> GMRIPLVGKEPIEAEDMGFTLIHEHLRVFSEAVRYQWPHLYNEDEELRNAVNEVKRAMQFGVKTIVDPTVMGLGRDIRFMEKVVKTTGINLVAGTGIYIYVDLPFYFLNRSIDEIADLFIHDIKEGIQATSNKAGFVKIAADEPGIT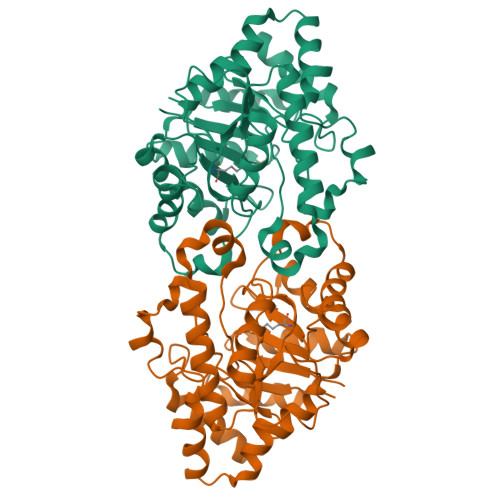KDVEKVIRAAAITHKEAKVPIITHSNAHNNTGLEEQRILMEEGVDPGKILIGHLGDTDNTDYIKKIADKGSFIGLDRYGLDLFLPVDKRNETTLKLIKDGYSDRIMISHDYCCTIDWGTARPELKPKLAPRWSMALIFEDTIPFLKKNGVSEEVIDIIFKENPKKFFS>SQSNRELVVDFLSYKLSQKGYSWSQFSDVEENRTEAPEETEAERETPSAINGNPSWHLADSPAVNGATGHSSSLDAREVIPMAAVKQALREAGDEFELRYRRAFSDLTSQLHITPGTAYQSFEQVVNELFRDGVNWGRIVAFF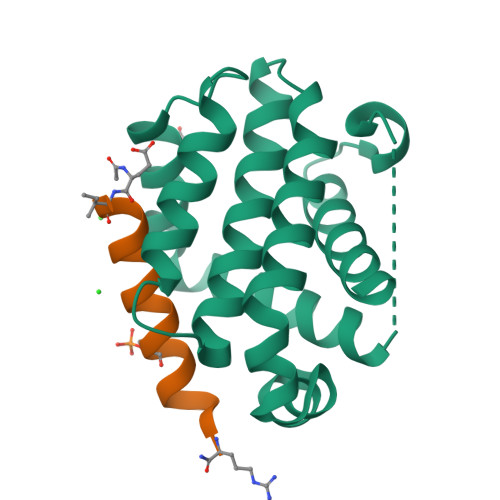SFGGALCVESVDKEMQVLVSRIASWMATYLNDHLEPWIQENGGWDTFVDLYG[2x];>XIWIAQELRSRGDSFNAYYAR[2x]> UUAAGUUAGGUUUGUGGUUGAAAGUCGAUGCCAGUCGCAGGCAAAACGAUCCACGUAAGUUAAACAAAGUUUUAAUGAGCAUGGUGCGGCUUAGAAGUAAGUCCUGCCGCUUUAGGCGAGAGUAUUAGUAGUGAGAGGGUAAUUCCGGGUAGCGAAACUUCCAGCAGGCGAGUGUGGGGU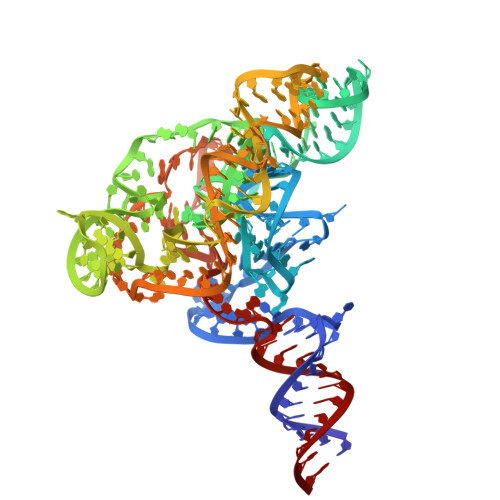CAAAGACCAGGUCAACUAACUUAA> MSSLSDQLAQVASNNATVALDRKRRQKLHSASLIYNSKTAATQDYDFIFENASKALEELSQIEPKF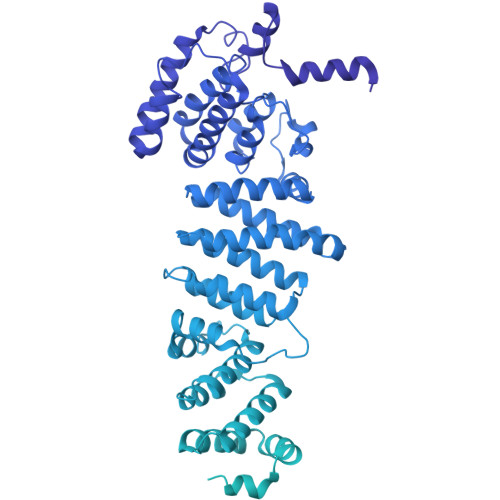AIFSRTLFSESSISLDRNVQTKEEIKDLDNAINAYLLLASSKWYLAPTLHATEWLVRRFQIHVKNTEMLLLSTLNYYQTPVFKRILSIIKLPPLFNCLSNFVRSEKPPTALTMIKLFNDMDFLKLYTSYLDQCIKHNATYTNQLLFTTCCFINVVAFNSNNDEKLNQLVPILLEISAKLLASKSKDCQIAAHTILVVFATALPLKKTIILAAMETILSNLDAKEAKHSALLTICKLFQTLKGQGNVDQLPSKIFKLFDSKFDTVSILTFLDKEDKPVCDKFITSYTRSIARYDRSKLNIILSLLKKIRLERYEVRLIITDLIYLSEILEDKSQLVELFEYFISINEDLVLKCLKSLGLTGELFEIRLTTSLFTNADVNTDIVKQLSDPVETTKKDTASFQTFLDKHSELINTTNVSMLTETGERYKKVLSLFTEAIGKGYKASSFLTSFFTTLESRITFLLRVTISPAAPTALKLISLNNIAKYINSIEKEVNIFTLVPCLICALRDASIKVRTGVKKILSLIAKRPSTKHYFLSDKLYGENVTIPMLNPKDSEAWLSGFLNEYVTENYDISRILTPKRNEKVFLMFWANQALLIPSPYAKTVLLDNLNKSPTYASSYSSLFEEFISHYLENRSSWEKSCIANKTNFEHFERSLVNLVSPKEKQSFMIDFVLSALNSDYEQLANIAAERLISIFASLNNAQKLKIVQNIVDSSSNVESSYDTVGVLQSLPLDSDIFVSILNQNSISNEMDQTDFSKRRRRRSSTSKNAFLKEEVSQLAELHLRKLTIILEALDKVRNVGSEKLLFTLLSLLSDLETLDQDGGLPVLYAQETLISCTLNTITYLKEHGCTELTNVRADILVSAIRNSASPQVQNKLLLVIGSLATLSSEVILHSVMPIFTFMGAHSIRQDDEFTTKVVERTILTVVPALIKNSKGNEKEEMEFLLLSFTTALQHVPRHRRVKLFSTLIKTLDPVKALGSFLFLIAQQYSSALVNFKIGEARILIEFIKALLVDLHVNEELSGLNDLLDIIKLLTSSKSSSEKKKSLESRVLFSNGVLNFSESEFLTFMNNTFEFINKITEETDQDYYDVRRNLRLKVYSVLLDETSDKKLIRNIREEFGTLLEGVLFFINSVELTFSCITSQENEEASDSETSLSDHTTEIKEILFKVLGNVLQILPVDEFVNAVLPLLSTSTNEDIRYHLTLVIGSKFELEGSEAIPIVNNVMKVLLDRMPLESKSVVISQVILNTMTALVSKYGKKLEGSILTQALTLATEKVSSDMTEVKISSLALITNCVQVLGVKSIAFYPKIVPPSIKLFDASLADSSNPLKEQLQVAILLLFAGLIKRIPSFLMSNILDVLHVIYFSREVDSSIRLSVISLIIENIDLKEVLKVLFRIWSTEIATSNDTVAVSLFLSTLESTVENIDKKSATSQSPIFFKLLLSLFEFRSISSFDNNTISRIEASVHEISNSYVLKMNDKVFRPLFVILVRWAFDGEGVTNAGITETERLLAFFKFFNKLQENLRGIITSYFTYLLEPVDMLLKRFISKDMENVNLRRLVINSLTSSLKFDRDEYWKSTSRFELISVSLVNQLSNIENSIGKYLVKAIGALASNNSGVDEHNQILNKLIVEHMKASCSSNEKLWAIRAMKLIYSKIGESWLVLLPQLVPVIAELLEDDDEEIEREVRTGLVKVVENVLGEPFDRYLD> MDKYDKNVPSDYDGLFQKAADANGVSYDLLRKVAWTESRFVPTAKSKTGPLGMMQFTKATAKALGLRVTDGPDDDRLNPELAINAAAKQLAGLVGKFDGDELKAALAYNQGEGRLGNPQLEAYSKGDFASISEEGRNYMRNLLDVAKSPMAGQLETFGGITPKGKGIPAEVGLAGIGHKQKVTQELPESTSFDVKGIEQEATAKPFAKDFWETHGETLDEYNSRSTFFGFKNAAEAELSNSVAGMAFRAGRLDNGFDVFKDTITPTRWNSHIWTPEELEKIRTEVKNPAYINVVTGGSPENLDDLIKLANENFENDSRAAEAGLGAKLSAGIIGAGVDPLSYVPMVGVTGKGFKLI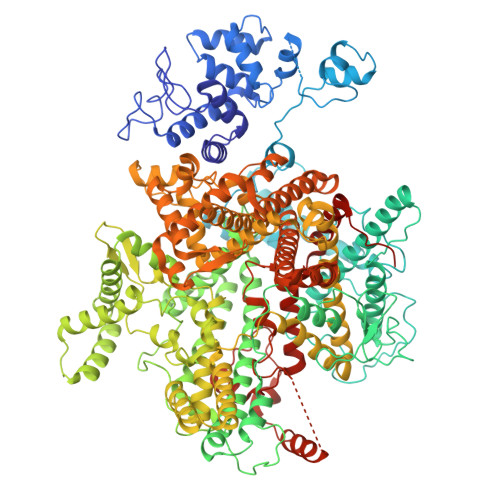NKALVVGAESAALNVASEGLRTSVAGGDADYAGAALGGFVFGAGMSAISDAVAAGLKRSKPEAEFDNEFIGPMMRLEARETARNANSADLSRMNTENMKFEGEHNGVPYEDLPTERGAVVLHDGSVLSASNPINPKTLKEFSEVDPEKAARGIKLAGFTEIGLKTLGSDDADIRRVAIDLVRSPTGMQSGASGKFGATASDIHERLHGTDQRTYNDLYKAMSDAMKDPEFSTGGAKMSREETRYTIYRRAALAIERPELQKALTPSERIVMDIIKRHFDTKRELMENPAIFGNTKAVSIFPESRHKGTYVPHVYDRHAKALMIQRYGAEGLQEGIARSWMNSYVSRPEVKARVDEMLKELHGVKEVTPEMVEKYAMDKAYGISHSDQFTNSSIIEENIEGLVGIENNSFLEARNLFDSDLSITMPDGQQFSVNDLRDFDMFRIMPAYDRRVNGDIAIMGSTGKTTKELKDEILALKAKAEGDGKKTGEVHALMDTVKILTGRARRNQDTVWETSLRAINDLGFFAKNAYMGAQNITEIAGMIVTGNVRALGHGIPILRDTLYKSKPVSAKELKELHASLFGKEVDQLIRPKRADIVQRLREATDTGPAVANIVGTLKYSTQELAARSPWTKLLNGTTNYLLDAARQGMLGDVISATLTGKTTRWEKEGFLRGASVTPEQMAGIKSLIKEHMVRGEDGKFTVKDKQAFSMDPRAMDLWRLADKVADEAMLRPHKVSLQDSHAFGALGKMVMQFKSFTIKSLNSKFLRTFYDGYKNNRAIDAALSIITSMGLAGGFYAMAAHVKAYALPKEKRKEYLERALDPTMIAHAALSRSSQLGAPLAMVDLVGGVLGFESSKMARSTILPKDTVKERDPNKPYTSREVMGAMGSNLLEQMPSAGFVANVGATLMNAAGVVNSPNKATEQDFMTGLMNSTKELVPNDPLTQQLVLKIYEANGVNLRERRK>[2x]GAMVNLRSLLVNPEGPTLMRLNSVQSSERPLFLVHPIEGSTTVFHSLASRLSIPTYGLQCTRAAPLDSIHSLAAYYIDCIRQVQPEGPYRVAGYSYGACVAFEMCSQLQAQQSPAPTHNSLFLFDGSPTYVLAYTQSYRAKLTPGCEAEAETEAICFFVQQFTDMEHNRVLEALLPLKGLEERVAAAVDLIIKSHQGLDRQELSF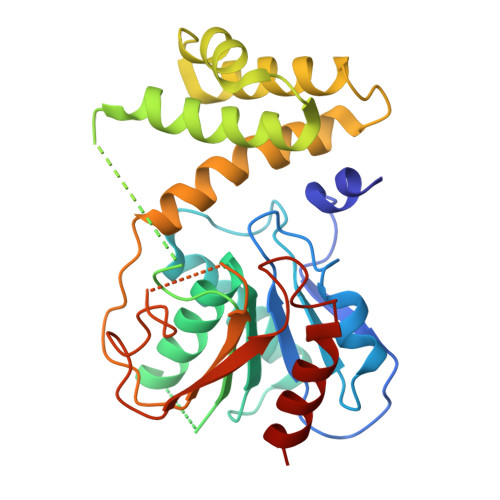AARSFYYKLRAAEQYTPKAKYYGNVMLLRAKTGGAYGEDLGADYNLSQVCDGKVSVHVIEGDHRTLLEGSGLESIISIIHSSLA>[3x]MELPADALPGEGAVREVLRPLLKQAAEKTAAGKIVFAEAATGTGKGRMIASLAAAAAIKGDTVVVSAPLAVTWQLVNDMKDIPEVRRVGLTLSLGRPNFISPQRTLEWAIDNERADLAAWIEGGGKPLSLRSMETSKVISHELCWLLEDALLLAEDLPADSLLLTSEDPADCPAQQLYVAMRSNYTEAGIILCSHFMLAAHTRMMQMRGLGNDEELDDEAPTGLSLPHFIDTLIVDEAHLLEQAFASVYTHTLRLRPLMRTIEGLGSRGRKPALDALKELFTQMQVASARSTNTSLNVPLSDVPELIPALKDTVKTLGALPTKGMSRDARSVIRIATRAANDALSGHSRLRIEVTPVHSYPMLLSGRSNLQRALLGLWNATGGATLVSATLFTTGDNGSLTRWKLEVPTERAAFLPPVHPAWTTAPVLLHKEFCAHEPDDSPEWATECAQTIQGVASTAQGGTLVLCTSYQNTELLAGRLGAALGDRLIVQSKTSSAATCLAQF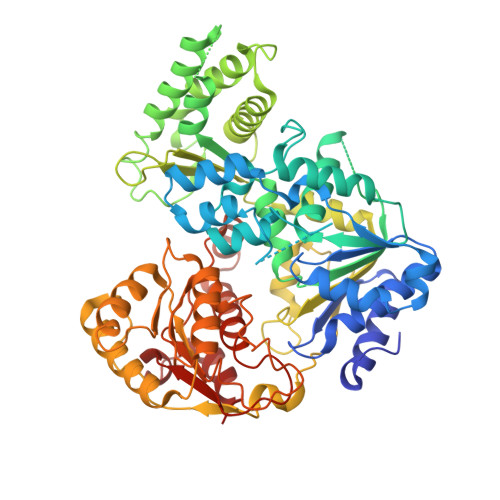KAKHKAGIRPVWLGLGAAWTGIDLSDHSLPDNPELDRLLSDLVITRIPVGQNRSLTHERRTAIGGFRIISQEAAWHFRQGLGRLVRRPGVTHKNLWVLDARIYGGAAWVAPFRQILDRYKKA>[2x]I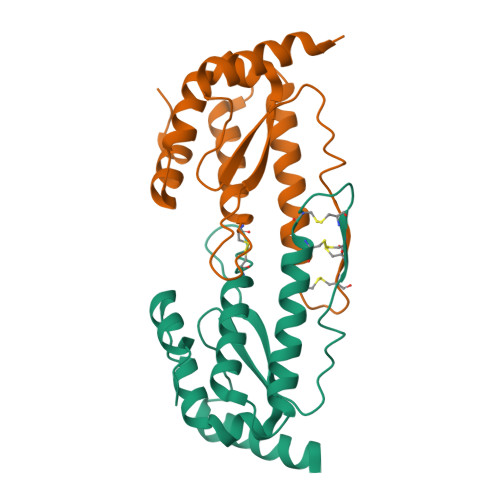NSLEELAAQELIAAQFEGNLDGFFCTFYVQSKPQLLDLESECYCMDDFDCGCDRIKREEELRKLIFLTSDVYGYNFEEWKGLVWKFVQNYCPEHRYGSTFGNGLLIVSPRFFMDHLDWFQQWKLVSSNDECRAFLRKRTQ> MVANPEHYIKHPLQNRWALWFFKNDKSKTWQANLRLISKFDTVEDFWALYNHIQLSSNLMPGCDYSLFKDGIEPMWEDEKNKRGGRWLITLNKQQRRSDLDRFWLETLLCLIGESFDDYSDDVCGAVVNVRA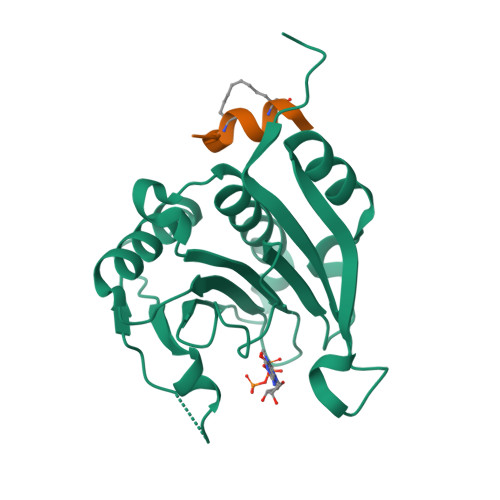KGDKIAIWTTECENREAVTHIGRVYKERLGLPPKIVIGYQSHADTATKSGSTTKNRFVV;> XKKRYSRLQLLLFWX> QPEQKASNLIGTYRHVD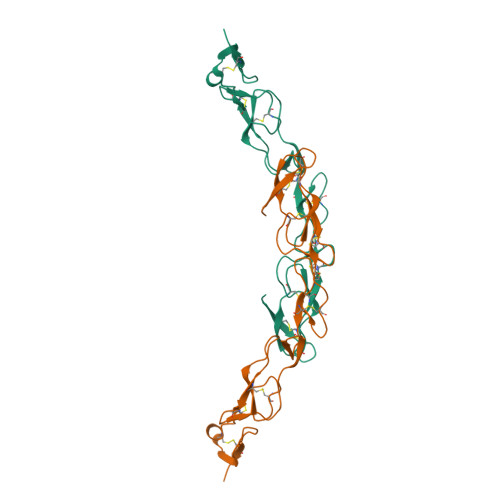RATGQVLTCDKCPAGTYVSEHCTNTSLRVCSSCPVGTFTRHENGIEKCHDCSQPCPWPMIEKLPCAALTDRECTCPPGMFQSNATCAPHTVCPVGWGVRKKGTETEDVRCKQCARGTFSDVPSSVMKCKAYTDCLSQNLVVIKPGTKETDNVCGTLPSFSSSTSPSPGTAIFPRPEHMETHEVPSSTYVPKGMNSTESNSSASVRPKVLSSIQEGTVPDNTSSARGKEDVNKTLPNLQVVNHQQGPHHRHILKLLPSMEATGGEKSSTPIKGPKRGHPRQNLHKHFDINEHHHHHH> MASEAKQTVHTGNTVLLMIKGKPVGRAQSASGQREYGTTGVYEIGSIMPQEHVYLRYEGTITVERLRMKKEN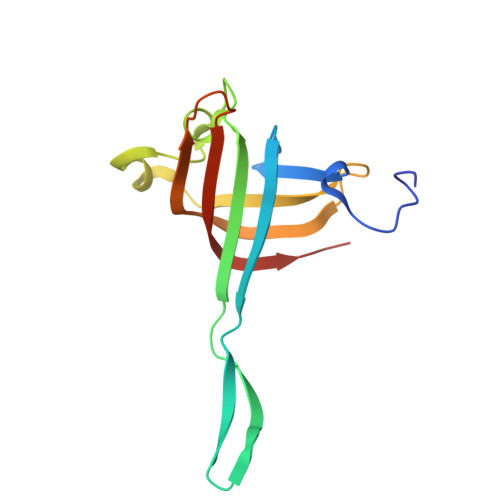FADLGYASLGEEILKKDIIDILVVDNLTKQVIISYHGCSANNYNETWQTNEIVTEEIEFSYLTASDKART> RMKGSKEVFLVKFVKSSGSSEYFLKALESIKEFQSEEHLQILEEEAALNIKENDKSLYICDPFTGVVFNH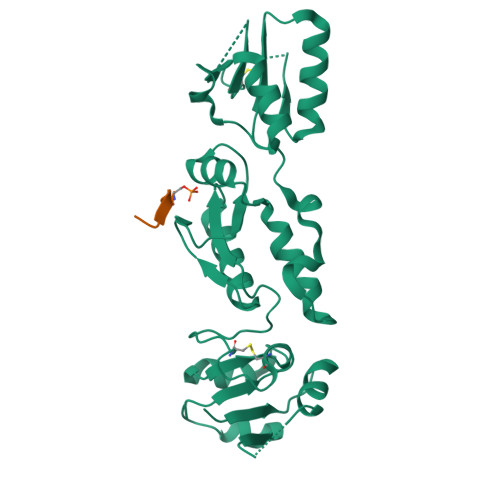LKKLGCRIVGPQVVLYCMQSQRCVPRAEYPVYNMTMADVTISCTTLDKDVREEVHKYVQMMGGRVYRDLNMSVTHLIAGEVGSKKYLVAASLKKPVLLPSWVKTLWDKSQQRMMRYTDVNMEDYACPVFLGCTICVTGLSSSDRKEVQRLTAEHGGQYSGQLKMNECTHLIVQEPKGQKYECAKKWNVHCVPVQWFSDSIEKGFCQDETMYKIESGSKLS;> SPVLAEDSEGE>QMPKTLRIRNGDKVRSTFSAQEYANRQARLRAHLAAENIDAAIFTSYHNINYYSDFLYCSFGRPYALVVTEDDVISISANIDGGQPWRRTVGTDNIVYTDWQRDNYFAAIQQALPKARRIGIEHDHLNLQNRDKLAARYPDAELVDVAAACMRMRMIKSAEEHVMIRHGARIADIGGAAVVEALGDQVPEYEVALHATQAMVRAIADTFEDVELMDTWTWFQSGINTDGAHNPVTTRKVNKGDILSLNCFPMIAGYYTALERTLFLDHCSDDHLRLWQ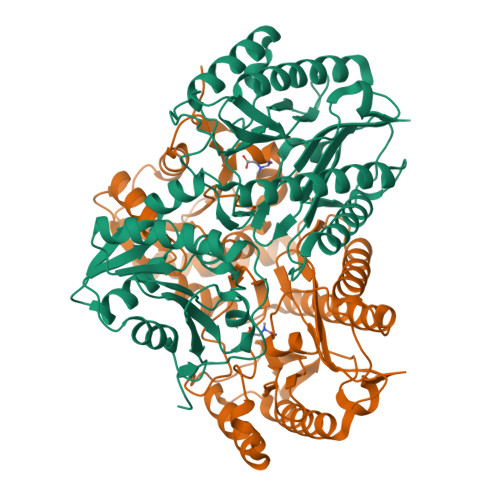VNVEVHEAGLKLIKPGARCSDIARELNEIFLKHDVLQYRTFGYGHSFGTLSHYYGREAGLELREDIDTVLEPGMVVSMEPMIMLPEGLPGAGGYREHDILIVNENGAENITKFPYGPEKNIIR[2x]>MEISELEGKKVPHGEVTLVGAGRLGFRTALNLMQIHRGGPERIKVIDGQKVSADDLIFRLMGAKIGEYKVKFIESLACDGFSRTVQGIPEYITGDNLRLIGGDVVCVEIAGGDTLPITTEIIRYAQERGAATISTMGVFGIGEEDVSVVDIDEADPENPIAA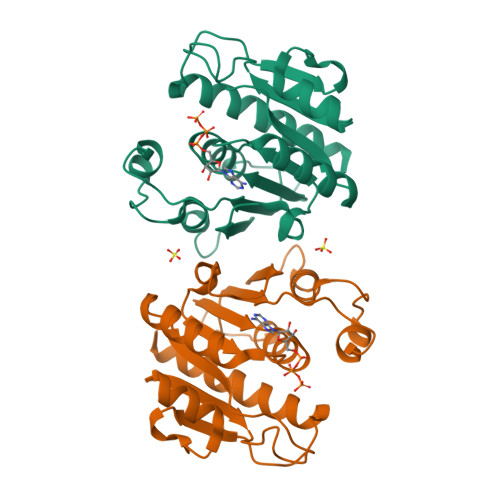YLQAEGIHEHVLVGTGKLIRDWEPVTPHVLDRVSEVMTAEILKLLRGAQRLELVPR[2x]> GAMGWEKAYRIKKNADFQRIYKKGHSVANRQFVVYTCNNKEIDHFRLGISVSKKLGNAVLRNKIKRAIRENFK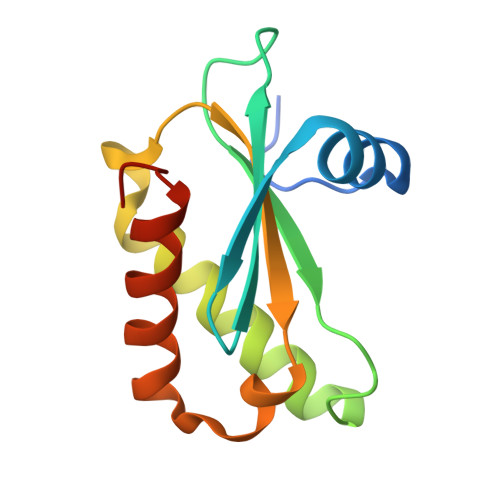VHKSHILAKDIIVIARQPAKDMTTLQIQNSLEHVLKIAKVFNKKIK>MDAEGLALLLPPVTLAALVDSWLREDCPGLNYAALVSGAGPSQAALWAKSPGVLAGQPFFDAIFTQLNCQVSWFLPEGSKLVPVARVAEVRGPAHCLLLGERVALNTLARCSGIASAAAAAVEAARGAGWTGHVAGTRKTTPGFRLVEKYGLLVGGAASHRYDLGGLVMVKDNHVVAAGGVEKAVRAARQAADFTLKVEVECSSLQEAVQAAEAGADLVLLDNFKPEELHPTATVLKAQFPSVAVEASGGITLDNLPQFCGPHIDVISMGMLTQAAPALDFSLKLFAKEVAPVPKIHLEHHHHHH[6x]

QPRTs have been shown to exist as dimers or hexamers2223242526272829. HsQPRT is regulated by the interaction between two dimeric subunits. which can adopt open and closed states.

nearly the same in both the apo form and the substrate complexes. conformation even though the apo form, which may hinder QA accessibility. that QA binds to hexameric apo HsQPRT with positive cooperativity.>[2x]MSMDISDFYQTFFDEADELLADMEQHLLVLQPEAPDAEQLNAIFRAAHSIKGGAGTFGFSVLQETTHLMENLLDEARRGEMQLNTDIINLFLETKDIMQEQLDAYKQSQE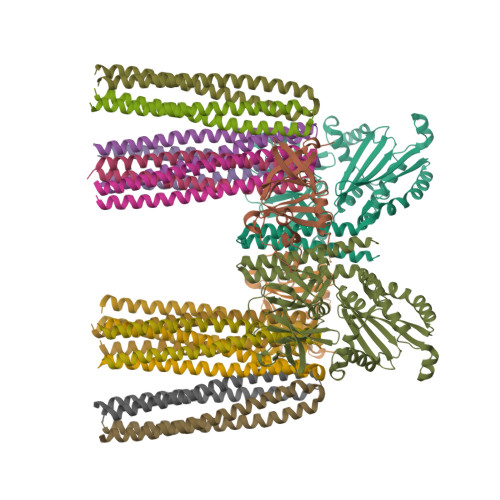PDAASFDYICQALRQLALEAKGETPSAVTRLSVVAKSEPQDEQSRSQSPRRIILSRLKAGEVDLLEEELGHLTTLTDVVKGADSLSAILPGDIAEDDITAVLCFVIEADQITFETVEVSPKISTPPVLKLAAEQAPTGRVEREKTTRSNESTSIRVAVEKVDQLINLVGELVITQSMLAQRSSELDPVNHGDLITSMGQLQRNARDLQESVMSIRMMPMEYVFSRYPRLVRDLAGKLGKQVELTLVGSSTELDKSLIERIIDPLTHLVRNSLDHGIELPEKRLAAGKNSVGNLILSAEHQGGNICIEVTDDGAGLNRERILAKAASQGLTVSENMSDDEVAMLIFAPGFSTAEQVTDVSGRGVGMDVVKRNIQKMGGHVEIQSKQGTGTTIRILLPLTLAILDGMSVRVADEVFILPLNAVMESLQPREADLHPLAGGERVLEVRGEYLPIVELWKVFNVAGAKTEATQGIVVILQSGGRRYALLVDQLIGQHQVVVKNLESNYRKVPGISAATILGDGSVALIVDVSALQAINREQRMANTAA;>[2x]MTGMTNVTKLASEPSGQEFLVFTLGDEEYGIDILKVQEIRGYDQVTRIANTPAFIKGVTNLRGVIVPIVDLRIKFSQVDVDYNDNTVVIVLNLGQRVVGIVVDGVSDVLSLTAEQIRPAPEFAVTLSTEYLTGLGALGDRMLILVNIEKLLNSEEMALLDSAASEVA;>[12x]MLKRIKIVTSLLLVLAVFGLLQLTSGGLFFNALKNDKENFTVLQTIRQQQSTLNGSWVALLQTRNTLNRAGIRYMMDQNNIGSGSTVAELMESASISLKQAEKNWADYEALPRDPRQSTAAAAEIKRNYDIYHNALAELIQLLGAGKINEFFDQPTQGYQDGFEKQYVAYMEQNDRLHDIAVSDNNASYSQAMWILVGVMIVVLAVIFAVWFGIKASLVAPMNRLIDSIRHIAGGDLVKPIEVDGSNEMGQLAESLRHMQGELMRTVGDVRNGANAIYSGASEIATGNNDLSSRTEQQAASLEETAASMEQLTATVKQNAENARQASHLALSASETAQRGGKVVDNVVQTMRDISTSSQKIADIISVIDGIAFQTNILALNAAVEAARAGEQGRGFAVVAGEVRNLAQRSAQAAREIKSLIEDSVGKVDVGSTLVESAGETMAEIVSAVTRVTDIMGEIASASDEQSRGIDQVGLAVAEMDRVTQQNAALVEESAAAAAALEEQASRLTEAVAVFRIQQQQRETSAVVKTVTPAAPRKMAVADSEENWETF> MRGSHHHHHHIAASRLDEIMERGTLRVGTTGDYKPFSYRDPDGQYTGFDIDVAKSLAKSLGVKVEFVPTTWPTLMSDLQADKFDIAMGGVTVTPERQKKADFSDPYMTFGKTPLVRKEDADKFKSLEDINRPDVRVAVNPGGTNEKFAREHLKKAKITVYENNVEIFQEVASGRADVMI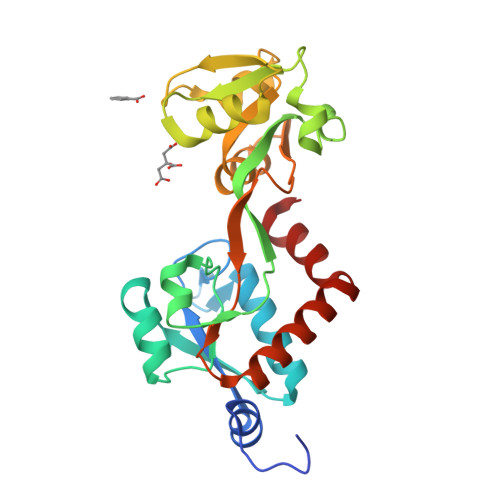TDTVEALYYAKKHPGLAAVLVDKPFTHSEKGYMMPKGDQEFLNYVNQWLDQMKQQGTYEKLYEKWLKL2-(2,4-dimethoxyphenyl)-1-{4-[(isoquinolin-5-yl)sulfonyl]piperazin-1-yl}ethan-1-one 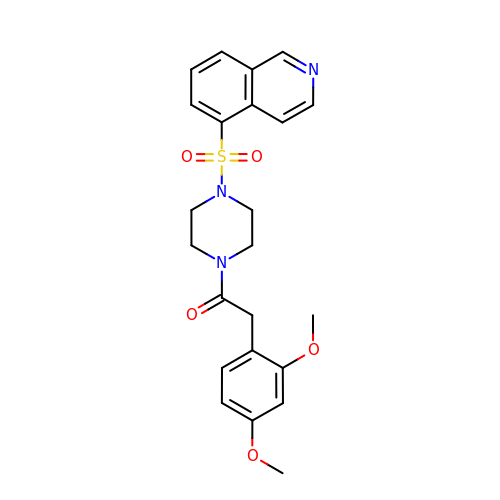| C23 H25 N3 O5 S | MEHDVSZDAVOOKI-UHFFFAOYSA-N>GVSEIRHTADRWRVSLDVNHFAPDELTVKTKDGVVEITGKHEERQDEHGYISRCFTRKYTLPPGVDPTQVSSSLSPEGTLTVEAPMP[8x];>[2x]ALSR;> LSGV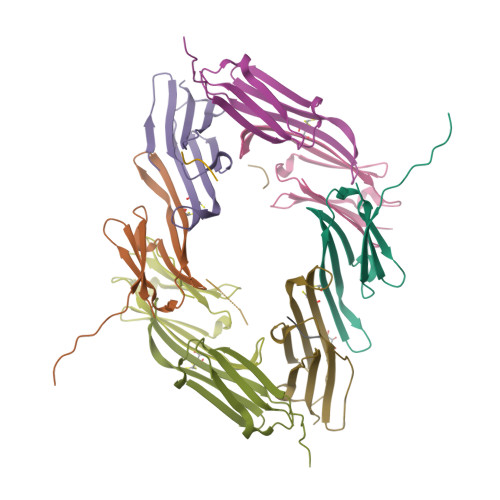;> ALSRQ>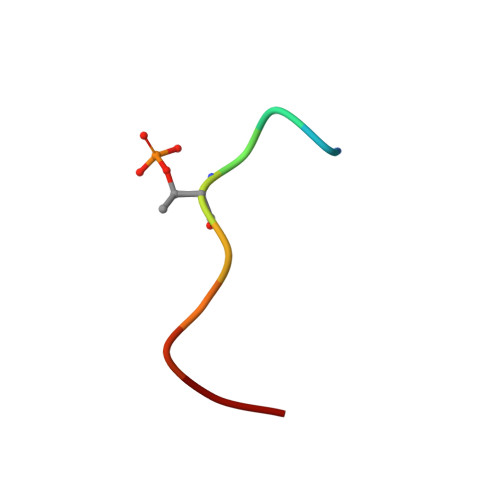 SIYFTPELYD> MARKFSSARPEMFRRFTPDSLEEIEAFTELKKSCTLEKKEPESTPRIDLEAGKPLPMIYGDPPEDLLNIPLEDLDPFYKTQKTFIVISKGNIINRFNAERALYIFSPFNPIRRGAIRVFVNSAFNFFIMFTIFSNCIFMTISNPPAWSKIVEYTFTGIYTFEVIVKVLSRGFCIGHFTFLRDPWNWLDFSVVTMTYITEFIDLRNVSALRTFRVLRALKTITIFPGLKTIVRALIESMKQMGDVVILTVFSLAVFTLAGMQLFMGNLRHKCIRWPISNVTLDYESAYNTTFDFTAYIENEENQYFLDGALDALLCGNNSDAGKCPEGYTCMKAGRNPNYGYTNYDNFAWTFLCLFRLMLQDYWENLYQMTLRAAGKSYMVFFIMVIFLGSFYLINLILAVVAMAYEEQNQATLAEAQEKEAEFQRAVEQLRIQQEQINDERKASLASQLTQNQEAEITDDGDDAIKECNGKAFPLANIREPSSVKLSTEEQRSDSKSMDSKHSVDKPSLKHKAASTMSVFTLEDLEAARRPCPPVWYKFAGFVFKWNCCGPWVFLKKWVHFVMMDPFTDLFITLCIILNTLFMSIEHHPMNESFQSLLSAGNLVFTTIFAAEMVLKIIALDPYYYFQQTWNIFDSIIVSLSLLELG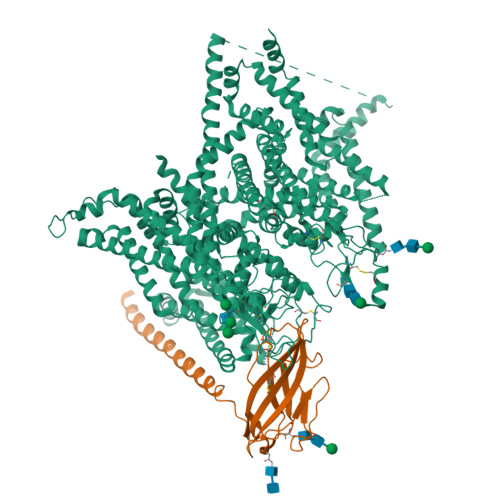LSNMQGMSVLRSLRLLRIFKLAKSWPTLNILIKIICNSVGALGNLTIVLAIIVFIFALVGFQLFGKNYKEYVCKISDDCELPRWHMNDFFHSFLIVFRALCGEWIETMWDCMEVGGVPMCLAVYMMVIIIGNLVMLNLFLALLLSSFSSDNLSSIEEDDEVNSLQVASERISRAKNWVKIFITGTVQALVLWIQGKKPPSDDVVGEEGDNEGKKDTLPLNYLDGEKIVDGITNCVESPTLNLPIVKGESEIEEEGLVDSSDEEDTNKKKHALNDEDSSVCSTVDYSPSEQDPLAKEEEEEEEEEPEELESKDPEACFTEKCIWRFPFLDVDITQGKGKIWWNLRRTCYTIVEHDYFETFIIFMILLSSGVLAFEDIYIWRRRVIKVILEYADKVFTYVFIVEMLLKWVAYGFKRYFTDAWCWLDFVIVGASIMGITSSLLGYEELGAIKNLRTIRALRPLRALSRFEGMKVVVRALLGAIPSIMNVLLVCLMFWLIFSIMGVNLFAGKFYRCINTTTDEILPVEEVNNRSDCMALMYTNEVRWVNLKVNYDNAGMGYLSLLQVSTFKGWMDIMYAAVDSREVEDQPIYEINVYMYLYFVIFIVFGAFFTLNLFIGVIIDNFNRQKQKLGGEDLFMTEEQKKYYNAMKKLGSKKAAKCIPRPSNVVQGVVYDIVTQPFTDIFIMALICINMVAMMVESEDQSQVKKDILSQINVIFVIIFTVECLLKLLALRQYFFTVGWNVFDFAVVVISIIGLLLSDIIEKYFVSPTLFRVIRLARIARVLRLIRAAKGIRTLLFALMMSLPALFNIGLLLFLIMFIFSIFGMSNFAYVKKQGGVDDIFNFETFGNSMICLFEITTSAGWDGLLLPTLNTGPPDCDPDVENPGTDVRGNCGNPGKGITFFCSYIILSFLVVVNMYIAIILENFGVAQEESSDLLCEDDFVMFDETWHKFDVHGTQFLDYNDLPRFVNALQEPMRIPNPNRHKLAKMDMYVVMEDKISYLDVLLAVTQEVLGDTTEMEAMRLSIQAKFKKDNPSPTFFEPVVTTLRRKEEEWASVVIQRAFRQYLLMRAVSHASFLSQIKHMNEGPKDGVGSQDSLITQKMNALYRGNPELTMPLEQQIKPMLDKPRMPSLSVPETYPIQIPKEVTNEVILHSAPMVRQNYSYSGAIVVRESIV;> MSAVQLLWMPVVLCVMQGRLSNGACVEVDSDTEAVVGHGFKLGCISCKMRGEVQASATVDWWFMAKGESEFSHIYSYIDMTGMVNDERFLDRLNWMGSKNTFDLQDGSIYILNVTLNDTGTYRCYFDRTLTFNYYEFRTNINKTITLNVVPKATRGTASILSEVMMYVSIIGLQLWLLVEMVYCYRKIAAAGEEALRESAAKPPLKLHP One example is the sperm-specific SLC9C1 that belongs to the SLC9 superfamily of cation/proton antiporters, known as Na+/H+ exchangers (NHEs), which are essential for the regulation of intracellular pH, sodium homeostasis and cell volume. The transport domain (TD) is accompanied by a voltage-sensing domain (VSD) and a cyclic-nucleotide binding domain (CNBD), which are regulatory units usually found in voltage-gated cyclic-nucleotide-modulated ion channels, also referred to as CNBD ion channels. In a recent patch-clamp fluorimetry study, the functional integrity of the domains was confirmed for SLC9C1 from the sea urchin Strongylocentrotus purpuratus, termed SpSLC9C1, identifying it as a Na+/H+ exchanger that is activated strictly by hyperpolarization and modulated by cyclic nucleotides (cNMPs). Specifically, SpSLC9C1 adapted to mediate cellular alkalization in sperm only in response to chemoattractant-induced hyperpolarization.

To investigate the impact of ligand binding on the conformation of SpSLC9C1, we solved the structures of the protein in the presence of cGMP and cAMP. In all cases, we could identify prominent densities within the CNBD corresponding to bound nucleotides, which were not present in the apo cryo-EM maps. Overall, the best-resolved cGMP- and cAMP-bound dimer structures, at 3.2 Å and 3.3 Å, respectively, share a similar conformation to the apo structure. However, we could identify key differences. Although image processing of the cGMP dataset revealed only one dominant conformation, the cAMP-bound dataset displayed a high degree of conformational heterogeneity throughout data analysis, and, in particular, the CTD was generally less resolved and mobile. In most of the three-dimensional (3D) classes and as observed in the 3D variability analysis, the dimer interaction between the β-CTDs is disrupted in the presence of cAMP, which causes the CTD to swing away from the symmetry axis. The observed flexibility in the CTD is also accompanied by a higher mobility of the VSDs, although at no point does the VSD approach the transport domain. Further, the extracellular tip of TM1 rotates around P75 towards the symmetry axis, pushing the TD protomers apart. Minor conformational differences between the three structures are β4 and β5 of the β-CNBD positioning closer to the bound nucleotides and a slight movement of helix C towards the β-CNBD in the cAMP-bound structure. Here, binding of cAMP causes the disruption of the dimer interface in the CTD, conferring it a higher mobility (state 4).

>[2x]MSKKRVVKLRELVPAVAALAVAVLIQSATGSSGGSGHTPTTQATHADDHDLTTHNGTEEHDDGHDDGHDDLHAHAPKVIVFISGSCLFGAISRSLFKKLPIPYTVVLLILGAILGVVASNVPLVEEHTRDVAHMDPHVLLQIFLPVLIFESAFAMDVHTFMRSFSQVCILALFGLVVASVLTAVLAMNLFNYNWNFSEAMMFGAIMSATDPVAVVALLKDLGASKQLGTIIEGESLLNDGCAIVIFNVFMKMVFFPQLTSTVGQNVLYFLQVAVAGPLWGYAVAKVTVFFLSHIFNDALVEITITLAATYLTYYIGDIWLEVSGVLAVVVLGLIVNAEKTSISPEVEVFLHRFWEMLAYLANTLIFMMVGVVVTQKALVAVDKMDWFYLIILYLAITIIRGMVISLFSPILSRIGYGLTWRNAVIMTWGGLRGAVGLALALVVENLAGNDVIGSKFLFHTAGIVVLTLVINATTIQTLLRILGMSDISIPKRLAMAGAVRRIHEGQNRTLNMLKSDRFLADADWDIATAACEISDPYSALSDDENAPADELTLGERKSVCPGCKAMVPNEPSPREFADMMEEARLRMLKAEKISYWKQFEHGMLAREALRLLVQHAEVAADEKDQFILVDDLKKSWQIKGIYPWLKRKLEDLISEKKIAAIPMPKYKLGKLMYKICHHMAFEVTINIAIVLNIVPIIMEFVVQDKMASVSTMAAPGSTVSSEPSSLQKIEDALRISNYVFFVIYAIEAIVKILGLGRHYIVSHWNKFDAFILVVALVDIIIAETLLKGSITINLSSIKVVKLFRLLRGLRMLRLTKALIPKLILVVNGKINNQLSLGYDVGKGYIIGEEEVGKIIDRMVDNKKILRELKHISETGRLQVVKELGLLQREHPGIAVSVKTRQAIRTILNHSRETIHELQGAGLLDEMEAHKLELTVEIKMKRLMNAPSSIPPPPPENLLKNVSWLAGDMKLIDFIKARASLLHFDYGEVIVREGDESDGLFLIVSGLVKLYGKSAFLDHDNPPVTAGSEENEVFEDYLTVGNVIGEMGVLTKKPRNATVTCETTVQVYFITAEDMNIAIDTFTLYPSLEYRLWRVVAIRIATPLIMEQMAFQGWTQEKVKLHLERGYLVDLAESHFQFNIDATLEDVILINGTAYNAHTREEIRSPCLISRTVHKLTFQYTATEEPRLFVVRNAEYNGPILDGRLDVDSKRSLISITEISSNMCLKHAAELRQKNSKVMLSRKSSGAAAKEEEDCIPNTSDVEQAAGVSPSVPTKTTPKPKSFLPSLGLSMSKERVNGEAVEESPVKTKQGEETPETEEGAAPRVNVALEVLFQ The polymerase is a multifunctional enzyme that is responsible for transcribing the viral negative sense RNA genome to generate polyadenylated mRNAs with a 5′ methylguanosine cap and replicating it to generate new viral genomes. The L protein contains three enzymatic domains: an RNA-dependent RNA polymerase (RdRp), a polyribonucleotidyltransferase (PRNTase), which is involved in cap addition, and a methyltransferase (MTase) that methylates the cap. Here we report a conserved allosteric inhibitory site identified on the L polymerase proteins of RSV and HMPV that can be targeted by a dual-specificity, non-nucleoside inhibitor, termed MRK-1. Functional analyses indicate that MRK-1 inhibits conformational changes necessary for the polymerase to engage in RNA synthesis initiation and to transition into an elongation mode.

Based on previous reports showing that the RSV CD, MTase, and CTD were disordered, a reductionist strategy was devised in which the L protein was truncated to remove these domains, with the rationale that their removal might aid particle density and orientations. Ltrunc-P was readily amenable to addition of the MRK-1 ligand and a co-complex structure was solved at a resolution of 2.39 Å. Density corresponding to MRK-1 was identified in a pocket located within the PRNTase domain and formed by the conserved motifs B, D, and E. Phe1385 (motif E) undergoes a rotamer change to accommodate the fluorophenyl group of MRK-1 and make an edge-face pi interaction. The side chain of His1338 (motif D) also rotates nearly 90˚ to accommodate MRK-1. There are several key interactions between the ligand and RSV L. The hydrazide of MRK-1 forms hydrogen bonds with the backbone carbonyl of Ile1381 and the side chain of His1338. The 4-cyclopropoxy-3-methoxybenzoyl group lies on Val1384, while also contacting Pro1002, Gly1218 (motif A), and Arg1345. At the other end, the fluorophenyl group of MRK-1 sits in a hydrophobic pocket created by Ile1241, Ile1368, and Thr1365. The site of partial resistance to MRK-1, Ile1381, contacts the central pyridinyl ring of MRK-1. The MRK-1 pocket is largely pre-formed except for the rotation of Phe1385, indicating that inhibitors of this class may target a low energy state of the polymerase without induced fit.

> MGSDYKDHDGDYKDHDIDYKDDDDKGSGSLEVLFQGPMDPIINGNSANVYLTDSYLKGVISFSECNALGSYIFNGPYLKNDYTNLISRQNPLIEHMNLKKLNITQSLISKYHKGEIKLEEPTYFQSLLMTYKSMTSSEQIATTNLLKKIIRRAIEISDVKVYAILNKLGLKEKDKIKSNNGQDEDNSVITTIIKDDILSAVKDNQSHLKADKNHSTKQKDTIKTTLLKKLMCSMQHPPSWLIHWFNLYTKLNNILTQYRSNEVKNHGFTLIDNQTLSGFQFILNQYGCIVYHKELKRITVTTYNQFLTWKDISLSRLNVCLITWISNCLNTLNKSLGLRCGFNNVILTQLFLYGDCILKLFHNEGFYIIKEVEGFIMSLILNITEEDQFRKRFYNSMLNNITDAANKAQKNLLSRVCHTLLDKTVSDNIINGRWIILLSKFLKLIKLAGDNNLNNLSELYFLFRIFGHPMVDERQAMDAVKINCNETKFYLLSSLSMLRGAFIYRIIKGFVNNYNRWPTLRNAIVLPLRWLTYYKLNTYPSLLELTERDLIVLSGLRFYREFRLPKKVDLEMIINDKAISPPKNLIWTSFPRNYMPSHIQNYIEHEKLKFSESDKSRRVLEYYLRDNKFNECDLYNCVVNQSYLNNPNHVVSLTGKERELSVGRMFAMQPGMFRQVQILAEKMIAENILQFFPESLTRYGDLELQKILELKAGISNKSNRYNDNYNNYISKCSIITDLSKFNQAFRYETSCICSDVLDELHGVQSLFSWLHLTIPHVTIICTYRHAPPYIGDHIVDLNNVDEQSGLYRYHMGGIEGWCQKLWTIEAISLLDLISLKGKFSITALINGDNQSIDISKPIRLMEGQTHAQADYLLALNSLKLLYKEYAGIGHKLKGTETYISRDMQFMSKTIQHNGVYYPASIKKVLRVGPWINTILDDFKVSLESIGSLTQELEYRGESLLCSLIFRNVWLYNQIALQLKNHALCNNKLYLDILKVLKHLKTFFNLDNIDTALTLYMNLPMLFGGGDPNLLYRSFYRRTPDFLTEAIVHSVFILSYYTNHDLKDKLQDLSDDRLNKFLTCIITFDKNPNAEFVTLMRDPQALGSERQAKITSEINRLAVTEVLSTAPNKIFSKSAQHYTTTEIDLNDIMQNIEPTYPHGLRVVYESLPFYKAEKIVNLISGTKSITNILEKTSAIDLTDIDRATEMMRKNITLLIRILPLDCNRDKREILSMENLSITELSKYVRERSWSLSNIVGVTSPSIMYTMDIKYTTSTISSGIIIEKYNVNSLTRGERGPTKPWVGSSTQEKKTMPVYNRQVLTKKQRDQIDLLAKLDWVYASIDNKDEFMEELSIGTLGLTYEKAKKLFPQYLSVNYLHRLTVSSRPCEFPASIPAYRTTNYHFDTSPINRILTEKYGDEDIDIVFQNCISFGLSLMSVVEQFTNVCPNRIILIPKLNEIHLMKPPIFTGDVDIHKLKQVIQKQHMFLPDKISLTQYVELF;>[4x]MEKFAPEFHGEDANNRATKFLESIKGKFTSPKDPKKKDSIISVNSIDIEVTKESPITSNSTIINPTNETDDTAGNKPNYQRKPLVSFKEDPTPSDNPFSKLYKETIETFDNNEEESSYSYEEINDQTNDNITARLDRIDEKLSEILGMLHTLVVASAGPTSARDGIRDAMIGLREEMIEKIRTEALMTNDRLEAMARLRNEESEKMAKDTSDEVSLNPTSEKLNNLLEGNDSDNDLSLEDFKGENKYFQGHHHHHH>[2x]MSDPERRVRSTLKKVFGFDSFKTPLQESATMAVVKGNKDVFVCMPTGAGKSLCYQLPALLAKGITIVVSPLIALIQDQVDHLLTLKVRVSSLNSKLSAQERKELLADLEREKPQTKILYITPEMAASSSFQPTLNSLVSRHLLSYLVVDEAHCVSQWGHDFRPDYLRLGALRSRLGHAPCVALTATATPQVQEDVFAALHLKKPVAIFKTPCFRANLFYDVQFKELISDPYGNLKDFCLKALGQEADKGLSGCGIVYCRTREACEQLAIELSCRGVNAKAYHAGLKASERTLVQNDWMEEKVPVIVATISFGMGVDKANVRFVAHWNIAKSMAGYYQESGRAGRDGKPSWCRLYYSRNDRDQVSFLIRKEVAKLQEKRGNKASDKATIMAFDALVTFCEELGCRHAAIAKYFGDALPACAKGCDHCQNPTAVRRRLEALERSSSW

RECQL5 (also known as RECQ5) is a member of the RecQ family of helicases, which are highly conserved throughout evolution, and function in many diverse cellular processes with the role of maintaining genome integrity. Specific roles have been established for RECQL5 in almost every cellular process involving DNA, including transcription, replication, recombination, chromosomal segregation and DNA repair. The Zn2+-binding domain consists of a pair of long antiparallel α-helices (also known as the helical hairpin), followed by series of short helices and loops, from which a cluster of cysteine residues bind in a typical Cys4 tetrahedral arrangement to a single Zn2+ ion.

In an attempt to improve the diffraction properties of these crystals a new construct spanning residues 11–453 was produced and crystallization experiments were set up with and without nucleotides as above. In this case crystals were obtained in complex with the nucleotide ADP/Mg2+ in two different crystal forms, both of which diffract to significantly higher resolution (1.8 Å for the monoclinic crystals, and 2.0 Å for the triclinic). The ADP bound structures were solved by molecular replacement using the APO form as a search model, with two RECQL5 monomers in the asymmetric unit of the monoclinic crystals, and four copies in the triclinic crystals. In the ADP complex, the ADP moiety is bound in the active site, making extensive interactions with residues in the D1 domain, several of which belong to the conserved helicase motifs Q, I and II. More specifically the adenine base is sandwiched between the side chains of Phe 26 and Lys 30, making π–π stacking interactions with the former and van der Waals interactions with the aliphatic region of the latter. Gln 34 (the Q of the ‘Q motif’, also known as helicase motif 0), accepts and donates hydrogen bonds to the N6 and N7 nitrogen's respectively, conferring nucleotide specificity to the binding site. The α and β phosphates are bound in the classic Walker A or P-loop configuration (also known as helicase motif I), making hydrogen bonds to five successive main chain nitrogens, bounded on the far side by Lys 58. The binding site is completed by a number of bound waters and a hydrated Mg2+ ion, which is well defined in the electron density and makes a number of water mediated interactions with D157 and E158, and is suitably positioned to interact with oxygens from both the β and γ phosphates of ATP. On a local level, the residues forming the bulk of the nucleotide contacts from motif I undergo a significant helix to loop transition, exchanging several hydrogen bonds from canonical α helical hydrogen bonds, to phosphate oxygen contacts, with the entirety of residues 53–55 shifted significantly to accommodate the nucleotide.>[2x]GPHMASMTGGQQMGRGSEFMMNASTKFSDNYDVKEELGKGAFSVVRRCVHKTTGLEFAAKIINTKKLSARDFQKLEREARICRKLQHPNIVRLHDSIQEESFHYLVFDLVTGGELFEDIVAREFYSEADASHCIQQILESIAYCHSNGIVHRNLKPENLLLASKAKGAAVKLADFGLAIEVNDSEAWHGFAGT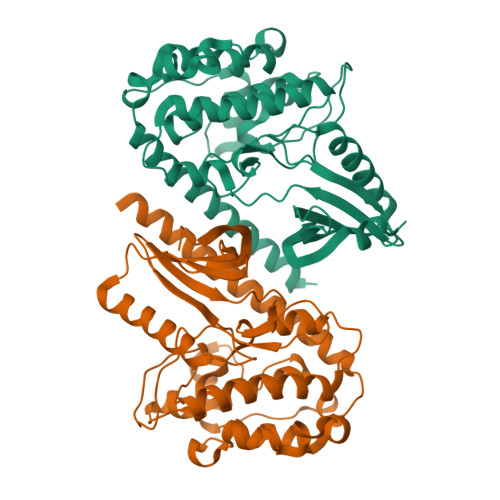PGYLSPEVLKKDPYSKPVDIWACGVILYILLVGYPPFWDEDQHRLYAQIKAGAYDYPSPEWDTVTPEAKSLIDSMLTVNPKKRITADQALKVPWICNRERVASAIHRQDTVDCLKKFNARRKLKGAILTTMIATRNLSNLGRNLLNKKEQGPPSTIKESSESSQTIDDN>MKASIALQVLPLVQGIDRIAVIDQVIAYLQTQEVTMVVTPFETVLEGEFDELMRILKEA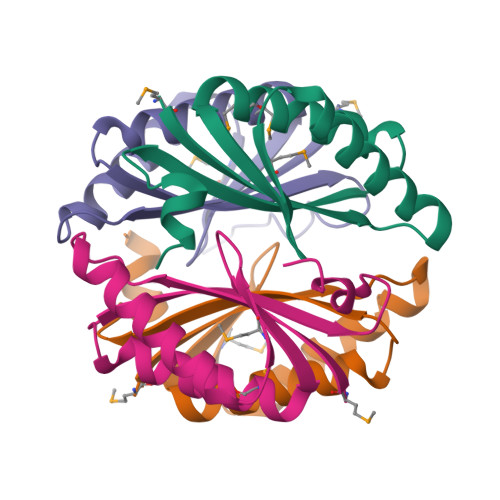LEVAGQEADNVFANVKINVGEILSIDEKLEKYTETTHLEHHHHHH[4x]>[2x]GHPLLDQRQPHYSAFGSVGEWLRAIKMGRYEESFAAA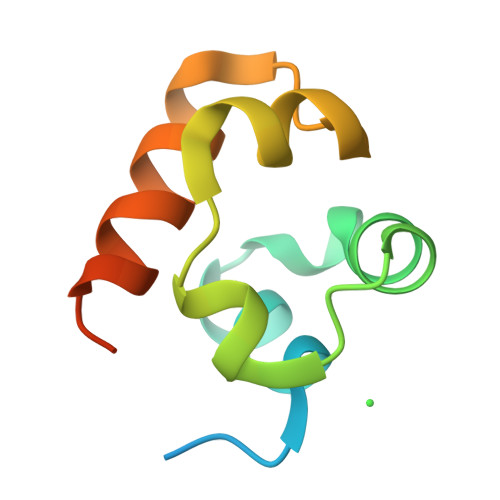GFGSFELVSQISAEDLLRIGVTLAGHQKKILASVQHMKSQAKPGTP> MSGTFHGDGHAPMSPFEDTFQFEDNSSNEDTHIAPTHFDDGATSNKYSRPQVSFNDETPKNKREDAEEFTFNDDTEYDNHSFQPTPKLNNGSGTFDDVELDNDSGEPHTNYDGMKRFRMGTKRNKKGNPIMGRSKTLKWARKNIPNPFEDFTKDDIDPGAINRAQELRTVYYNMPLPKDMIDEEGNPIMQYPRNKIRTTKYTPLTFLPKNILFQFHNFANVYFLVLIILGAFQIFGVTNPGLSAVPLVVIVIITAIKDAIEDSRRTVLDLEVNNTKTHILEGVENENVSTDNISLWRRFKKANSRLLFKFIQYCKEHLTEEGKKKRMQRKRHELRVQKTVGTSGPRSSLDSIDSYRVSADYGRPSLDYDNLEQGAGEANIVDRSLPPRTDCKFAKNYWKGVKVGDIVRIHNNDEIPADIILLSTSDTDGACYVETKNLDGETNLKVRQSLKCTNTIRTSKDIARTKFWIESEGPHSNLYTYQGNMKWRNLADGEIRNEPITINNVLLRGCTLRNTKWAMGVVMFTGGDTKIMLNSGITPTKKSRISRELNF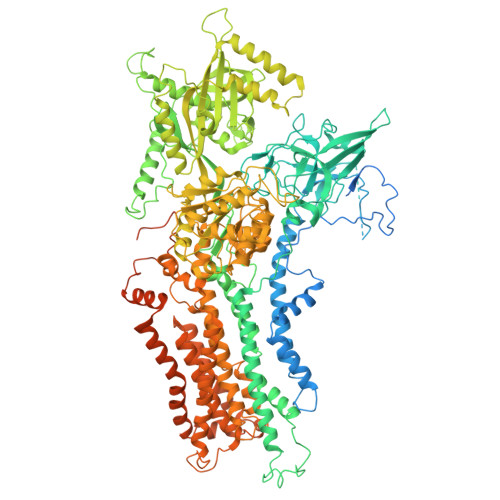SVVINFVLLFILCFVSGIANGVYYDKKGRSRFSYEFGTIAGSAATNGFVSFWVAVILYQSLVPISLYISVEIIKTAQAAFIYGDVLLYNAKLDYPCTPKSWNISDDLGQVEYIFSDKTGTLTQNVMEFKKCTINGVSYGRAYTEALAGLRKRQGIDVETEGRREKAEIAKDRDTMIDELRALSGNSQFYPEEVTFVSKEFVRDLKGASGEVQQRCCEHFMLALALCHSVLVEANPDNPKKLDLKAQSPDEAALVATARDVGFSFVGKTKKGLIIEMQGIQKEFEILNILEFNSSRKRMSCIVKIPGLNPGDEPRALLICKGADSIIYSRLSRQSGSNSEAILEKTALHLEQYATEGLRTLCIAQRELSWSEYEKWNEKYDIAAASLANREDELEVVADSIERELILLGGTAIEDRLQDGVPDCIELLAEAGIKLWVLTGDKVETAINIGFSCNLLNNEMELLVIKTTGDDVKEFGSEPSEIVDALLSKYLKEYFNLTGSEEEIFEAKKDHEFPKGNYAIVIDGDALKLALYGEDIRRKFLLLCKNCRAVLCCRVSPSQKAAVVKLVKDSLDVMTLAIGDGSNDVAMIQSADVGIGIAGEEGRQAVMCSDYAIGQFRYLARLVLVHGRWSYKRLAEMIPEFFYKNMIFALALFWYGIYNDFDGSYLYEYTYMMFYNLAFTSLPVIFLGILDQDVNDTISLVVPQLYRVGILRKEWNQRKFLWYMLDGLYQSIICFFFPYLVYHKNMIVTSNGLGLDHRYFVGVYVTTIAVISCNTYVLLHQYRWDWFSGLFIALSCLVVFAWTGIWSSAIASREFFKAAARIYGAPSFWAVFFVAVLFCLLPRFTYDSFQKFFYPTDVEIVREMWQHGHFDHYPPGYDPTDPNRPKVTKAGQHGEKIIEGIALSDNLGGSNYSRDSVVTEEIPMTFMHGEDGSPSGYQKQETWMTSPKETQDLLQSPQFQQAQTFGRGPSTNVRSSLDRTREQMIATNQLDNRYSVERARTSLDLPGVTNAASLIGTQQNN>SITDYNYKKPLHNDYQILDKSKIFGSNSGSFVMYSMAADAYYIYNEKESRKRYSPNSTYKIYLAMFGLDRHII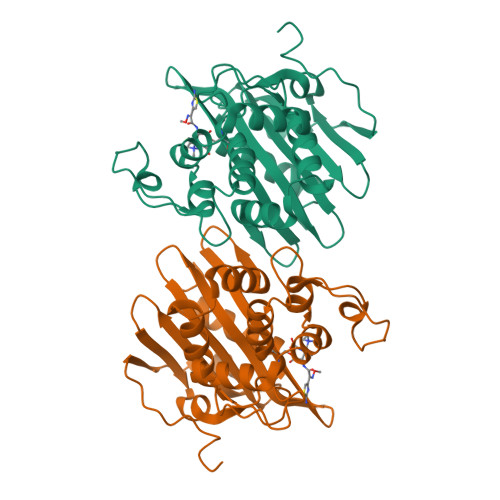NDENSRMSWNHKHYPFDAWNKEQDLNTAMQNSVNWYFERISDQIPKNYTATQLKQLNYGNKNLGSYKSYWMEDSLKISNLEQVIVFKNMMEQNNHFSKKAKNQLSSSLLIKKNEKYELYGKTGTGIVNGKYNNGWFVGYVITNHDKYYFATHLSDGKPSGKNAELISEKILKEMGVLN[2x]> HHHHHHMDIIFYHPTFDTQWWIEALRKAIPQARVRAWKSGDNDSADYALVFSPPVEMLAGRDLKAVFALGAGVDSILSKLQAHPEMLNPSVPLFRLEDTGMGEQMQEYAVSQVLHWFRRFDDYRIQQNSSHWQPLPEYHREDFTIGILGAGVLGSKVAQSLQTWRFPLRCWSRTRKSWPGVQSFAGREELSAFLSQCRVLINLLPNTPETVGIINQQLLEKLPDGAYLLNLARGVHVV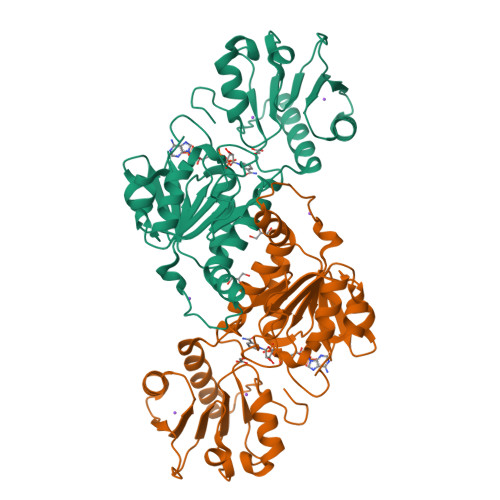EDDLLAALDSGKVKGAMLDVFNREPLPPESPLWQHPRVTITPHVAAITRPAEAVEYISRTIAQLEKGEKVCGQVDRARGY> MSDMNNPSDENTGALDDLWADALNEQKATTTKSAADAVFQQLGGGDVSGAMQDIDLIMDIPVKLTVELGRTRMTIKELLRLTQGSVVALDGLAGEPLDILINGYLIAQ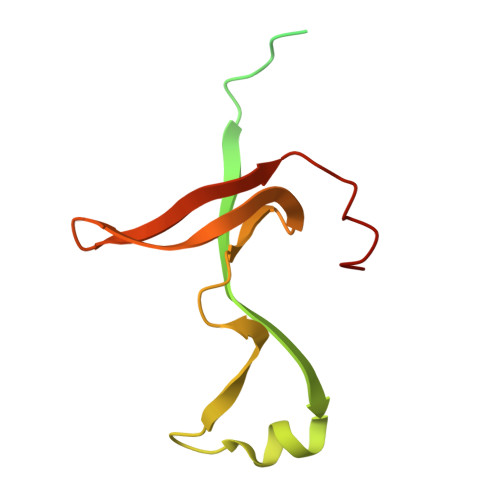GEVVVVADKYGVRITDIITPSERMRRLSR> MAFTIDFSDHTGLVKDAWYKQIEDLLEFAKKEEHIED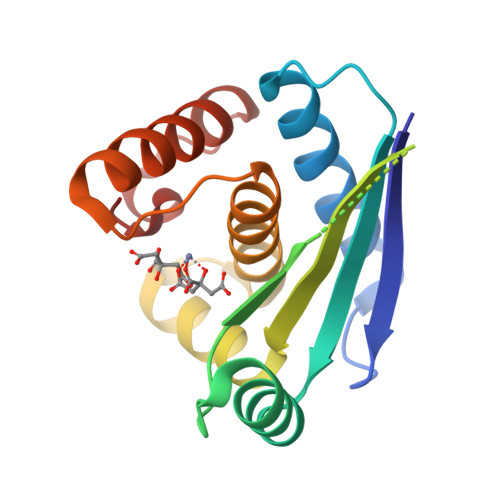DAELSVTFVDKQEIQEINRTYRDKDKVTDVISFALEEDEPEIDFSGLDIPRVLGDIIICTDVAQEQANNYGHSFERELGFLALHGFLHLLGYDHMTEADEKEMFGRQDTILNAYGLTRDHHHHHH>GARRFLCGVVEGFYGRPWVMEQRKELFRRLQKW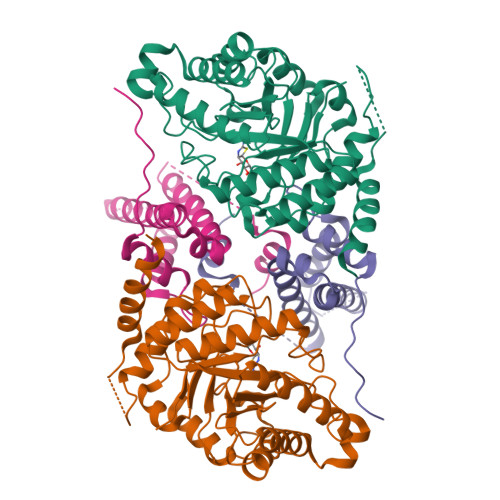ELNTYLYAPKDDYKHRMFWREMYSVEEAEQLMTLISAAREYEIEFIYAISPGLDITFSNPKEVSTLKRKLDQVSQFGCRSFALLFDDIDHNMCAADKEVFSSFAHAQVSITNEIYQYLGEPETFLFCPTEYCGTFCYPNVSQSPYLRTVGEKLLPGIEVLWTGPKVVSKEIPVESIEEVSKIIKRAPVIWDNIHANDYDQKRLFLGPYKGRSTELIPRLKGVLTNPNCEFEANYVAIHTLATWYKSNMNGVRKDVVMTDSEDSTVSIQIKLENEGSDEDIETDVLYSPQMALKLALTEWLQEFGVPHQYSSR[2x];>MEKPLYTAEPVTLEDLQLLADLFYLPYEHGPKGAQMLREFQWLRANSSVVSVNCKGKDSEKIEEWRSRAAKFEEMCGLVMGMFTRLSNCANRTILYDMYSYVWDIKSIMSMVKSFVQWLGCRSHSSAQFLIGDQEPWAFRGGLAGEFQRLLPIDGANDLFFQP[2x]> SNAMWETKFAKEGLTFDDVLLVPAKSDVLPNDVDLSVEMAPSLKLNVPIWSAGMDTITEAKMAIAIARQGGIGVVHKNMSIEQQAEEIEKVK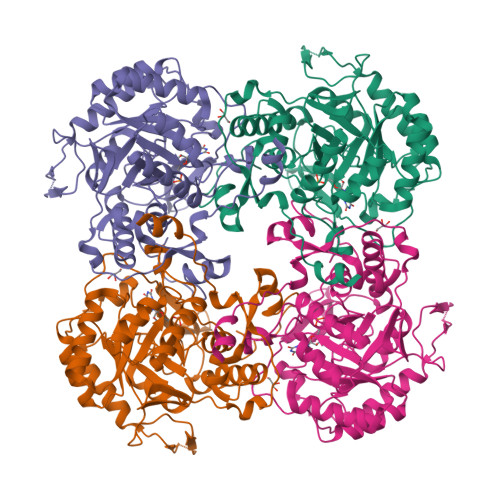RSESGGIKDIEKVIEFPNSAKDKHGRLLAAAAVGITNDTFVRVEKLIEAGVDAIVIDTAHGHSAGVINKISEIRQTFKDVVIVAGNVATAEGARALFEVGVDIVKVGIGPGSICTTRVVAGVGVPQITAIYDCATVAREFGKTIIADGGIKYSGDIVKALAAGGNAVMLGSMLAGTDESPGETEIFQGRQFKTYRGMGSLAAMEHGSKDRYFQADAKKLVPEGIEGRVPYKGSVADIIFQLVGGIRSGMGYTGSPDLRHLREEAAFVRMTGAGLRESHPHDIQITKEAPNYSIS>[2x]MDLFSVRMRAQKNGKHVSGAERIVKKEELETAVK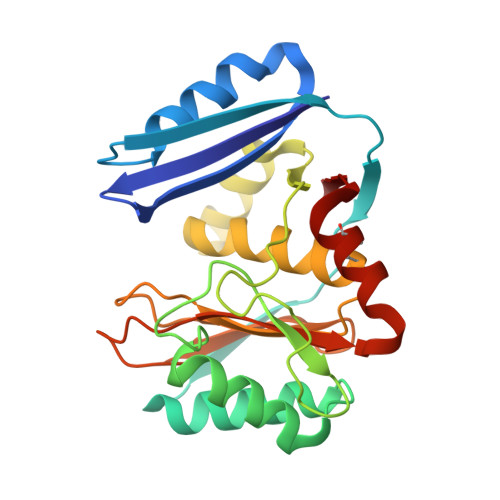ELLNRPKEFDFMNVKVEKVKDFEVVKFNLKISTYSFKSPEEAREFAVKKLTQEGIKEEVAKKAVEILSKGANPKGGNMRGAVLMDIETGERLEEDKERGVRTIHFDWKDRKKVTEKLLKEGYTLRTVDALALTFKNLFCGVVAELCWSDDPDYVTGYVSGKEIGYVRITPLKEKGDPLGGRVYFVSRKELSEIIECLTQKVVLIEL> SMSKSKDDAPHELESQFILRLPPEYASTVRRAVQSGHVNLKDRLTIELHPDGRHGIVRVDRVPLASKLVDLPCVMESLKTIDKKTFYKTADICQMLVSTVDGDLYPPVEEPVASTDPKASKKKDKDKEKKFIWNHGITLPLKNVRKRRFRKTAKKKYIESPDVEKEVKRLLSTDAEAVSTRWEIIAEDETKEAENQGLDISSPGMSGHRQGHDSLEHDELREIFNDLSSSSEDEDETQHQDEEDINIIDTEEDLERQLQDKLNESDEQHQENEGTNQLVMGIQKQIDNMKGKLQETQDRAKRQEDLIMKVENLALKNRFQAVLDELKQKEDREKEQL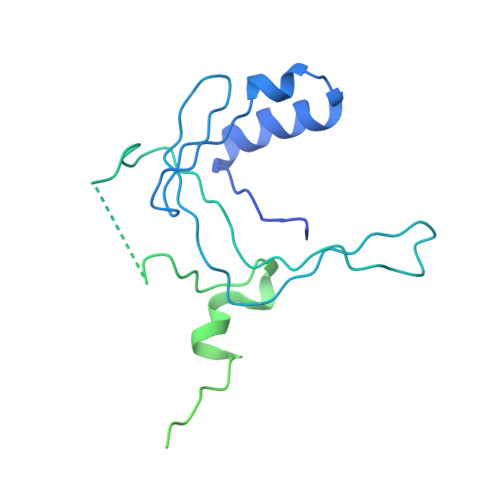SSLQEELESLLEK> MNEVIKSLTDHRS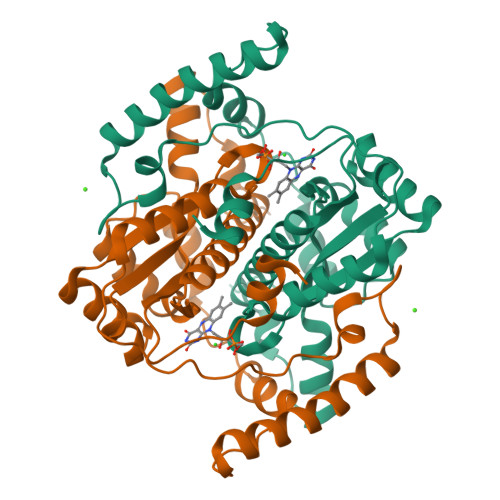IRSYTDEPVAQEQLDQIIEAVQSAPSSINGQQVTVITVQDKERKKKISELAGGQPWIDQAPVFLLFCADFNRAKIALEDLHDFKMEITNGLESVLVGAVDAGIALGTATAAAESLGLGTVPIGAVRGNPQELIELLELPKYVFPLSGLVIGHPADRSAKKPRLPQEAVNHQETYLNQDELTSHIQAYDEQMSEYMNKRTNGKETRNWSQSIASYYERLYYPHIREMLEKQGFKVEKHHHHHH2-OXOADIPIC ACID | C6 H8 O5 | 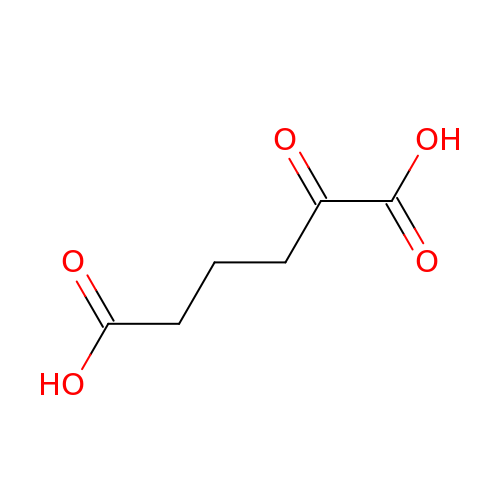FGSBNBBHOZHUBO-UHFFFAOYSA-N> MKKTWWKEGVAYQIYPRSFMDANGDGIGDLRGIIEKLDYLVELGVDIVWICPIYRSPNADNGYDISDYYAIMDEFGTMDDFDELLAQAHRRGLKVILDLVINHTSDEHPWFIESRSSRDNPKRDWYIWRDGKDGREPNNWESIFGGSAWQYDERTGQYYLHIFDVKQPDLNWENSEVRQALYEMVNWWLDKGIDGFRIDAISHIKKKPGLPDLPNPKGLKYVPSFAGHMNQPGIMEYLRELKEQTFARYDIMTVGEANGVTVDEAEQWVGEENGVFNMIFQFEHLGLWERRADGSIDVRRLKRTLTKWQKGLENRGWNALFLENHDLPRSVSTWGNDRDYWAESAKALGALYFFMQGTPFIYQGQEIGMTNVRFDDIRDYRDVSALRLYELERAKGRTHEEAMTIIWKTGRDNSRTPMQWS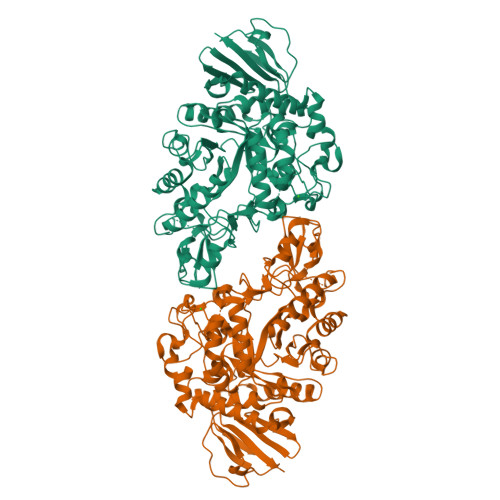GASNAGFTTGTPWIKVNENYRTINVEAERRDPNSVWSFYRQMIQLRKANELFVYGTYDLLLENHPSIYAYTRTLGRDRALVVVNLSDRPSLYRYDGFRLQSSDLALSNYPVRPHKNATRFKLKPYEARVYIWKE> GVINFSHADTYGNDSVGAHLQNVVYPTDAPFNAATDGTTDTTVAIKSAIAHCISKGKKLVLNHLFMITDTLVISDGLHVECLTSDSGVKSDVPAGKFAVKITGANSGWFGGKILGKNLPESTTVRQDGVLFDENAEYCFITGTEVTGFFAKGLHTSDADGVGYGIYDKGYGTLISKCYANSKFCVALGGTEGRVLKNRITNNYLTSGEAKPWSWASNYWDGIVSENAHRYVIAFNDVSACGQSGIYFGGNGGYSTDNIIVNNTVYACWNRGIDMGLFSEKSATNDVLRNIIKGNNTYNNRENNIWLAGVSNCSVVGNTSWFDTNYDVIFAGYPGGHICISLASGANGEACVGNTIDSNTCIDPRGNAGITVPTGATGNVFGSGNNLSQAGAIYIASPDLITSNRFELAVTGSFTPVLLPESGSITLSSSSTGVFRATGNRIDFSVTVNVSSISSPSGNLNIAYLPGMSGKTSSTSMFIIDYWNDLTL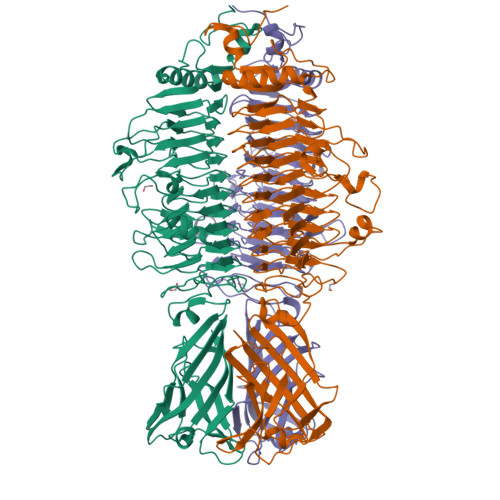SSGVIPLASLNLENQDQITVYRTDGGRVLYDFSSLMKSTSSFILKGFVDFN>[30x]GSHMKTENAKTITAVSSQHSADSKEKTAEVFKASKSDKPKDSIDD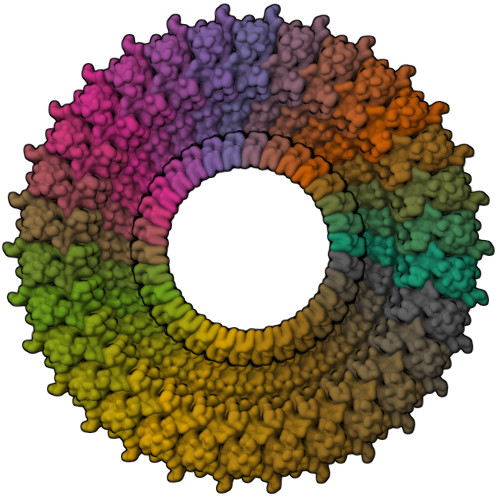YEKEYENQLKEILETIIGVDDVSVVVNVDATSLKVYEKNKSNKNTTTEETDKEGGKRSVTDQSSEEEIVMIKNGDKETPVVVQTKKPDIRGVLVVAQGVDNVQIKQTIIEAVTRVLDVPSHRVAVAPKKIKEDS>MASMAQTGTERVKRGMAEMQKGGVIMDVINAEQAKIAEEAGAVAVMALERVPADIRAAGGVARMADPTIVEEVMNAVSIPVMAKARIGHIVEARVLEAMGVDYIDESEVLTPADEEFHLNKNEYTVPFVCGCRDLGEA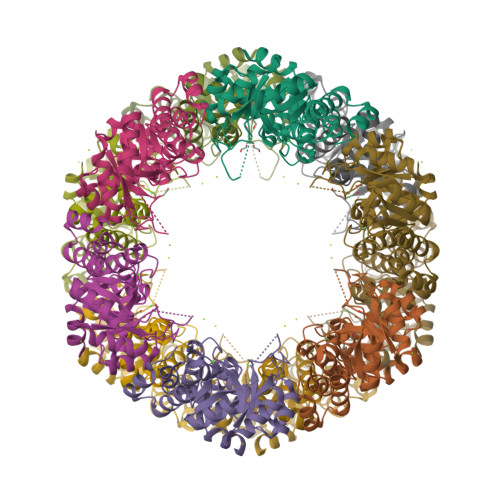TRRIAEGASMLRTKGEPGTGNIVEAVRHMRKVNAQVRKVVAMSEDELMTEAKNLGAPYELLLQIKKDGKLPVVNFAAGGVATPADAALMMQLGADGVFVGSGIFKSDNPAKFAKAIVEATTHFTDYKLIAELSKELGTAMKGIEISNLLPEQRMQERGWLEHHHHHH[6x]>MSQHNEKNPHQHQSPLHDSSEAKPGMDSLAPEDGSHRPAAEPTPPGAQPTAPGSLKAPDTRNEKLNSLEDVRKGSENYALTTNQGVRIADDQNSLRAGNRGPTLLEDFILREKITHFDHERIPERIVHARGSAAHGYFQPYKSLSDITKADFLSDPNKITPVFVRFSTVQGGAGSADTVRDIRGFATKFYTEEGIFDLVGNNTPIFFIQDAHKFPDFVHAVKPEPHWAIPQGQSAHDTFWDYVSLQ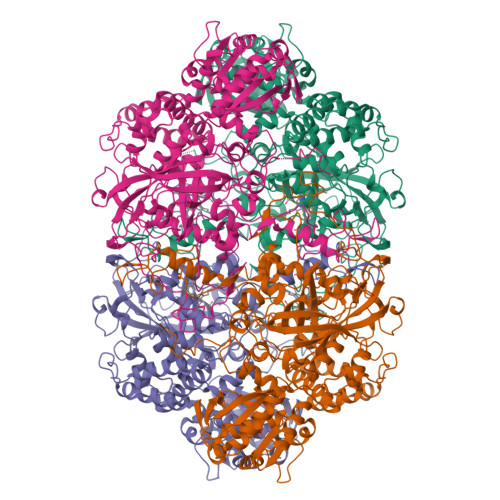PETLHNVMWAMSDRGIPRSYRTMEGFGIHTFRLINAEGKATFVRFHWKPLAGKASLVWDEAQKLTGRDPDFHRRELWEAIEAGDFPEYELGFQLIPEEDEFKFDFDLLDPTKLIPEELVPVQRVGKMVLNRNPDNFFAENEQAAFCPGHIVPGLDFTNDPLLQGRLFSYIDTQISRLGGPNFHEIPINRPTCPYHNFQRDGMHRMGIDTNPANYEPNSINDNWPRETPPGPKRGGFESYQERVEGNKVRERSPSFGEYYSHPRLFWLSQTPFEQRHIVDGFSFELSKVVRPYIRERVVDQLAHIDLTLAQAVAKNLGIELTDDQLNITPPPDVNSLKKDPSLSLYAIPDGDVKGRVVAILLNDEVRSADLLAILKALKAKGVHAKLLYSRMGEVTADDGTVLPIAATFAGAPSLTVDAVIVPCGNIADIADNGDANYYLMEAYKHLKPIALAGDARKFKATIKVADQGEEGIVEADSADGSFMDELLTLMAAHRVWSRIPKIDKIPA[4x]> LTAKHRPSVVWLHNAECTGCTEAAIRTIKPYIDALILDTISLDYQETIMAAAGEAAEAALHQALEGKDGYYLVVEGGLPTIDGGQWGMVAGHPMIETTKKAAAKAKGIICIGTCSAYGGVQKAKPNPSQAKGVSEALGVKTINIPGCPPNPINFVGAVVHVLTKGIPDLDSNGRPKLFYGELVHD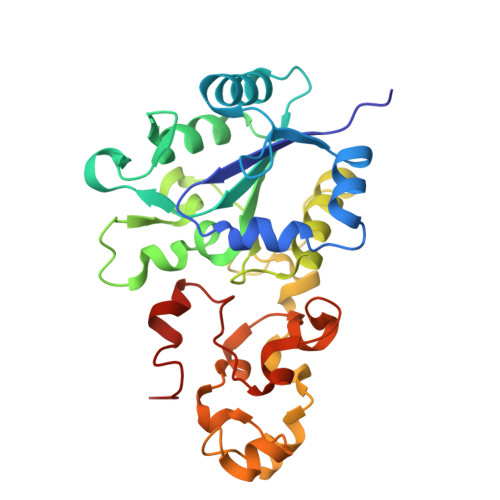NCPRLPHFEASEFAPSFDSEEAKKGFCLYELGCKGPVTYNNCPKVLFNQVNWPVQAGHPCLGCSEPDFWDTMTPFYEQG> MASAAVANYEEEIVRPVADFSPSLWGDQFLSFSIDNQVAEKYAQEIEALKEQTRSMLLATGRKLADTLNLIDIIERLGISYHFEKEIDEILDQIYNQNSNCNDLCTSALQFRLLRQHGFNISPEIFSKFQDENGKFKESLASDVLGLLNLYEASHVRTHADDILEDALAFSTIHLESAAPHLKSPLREQVTHALEQCLHKGVPRVETRFFISSIYDKEQSKNNVLLRFAKLDFNLLQMLHKQELAQVSRWWKDLDFVTTLPYARDRVVECYFWALGVYFEP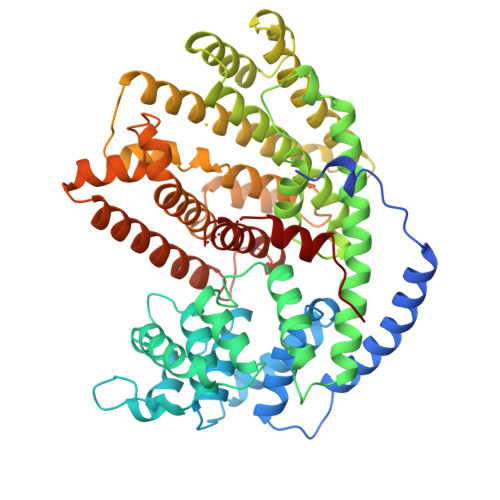QYSQARVMLVKTISMISIVDDTFDAYGTVKELEAYTDAIQRWDINEIDRLPDYMKISYKAILDLYKDYEKELSSAGRSHIVCHAIERMKEVVRNYNVESTWFIEGYTPPVSEYLSNALATTTYYYLATTSYLGMKSATEQDFEWLSKNPKILEASVIICRVIDDTATYEVEKSRGQIATGIECCMRDYGISTKEAMAKFQNMAETAWKDINEGLLRPTPVSTEFLTPILNLARIVEVTYIHNLDGYTHPEKVLKPHIINLLVDSIKI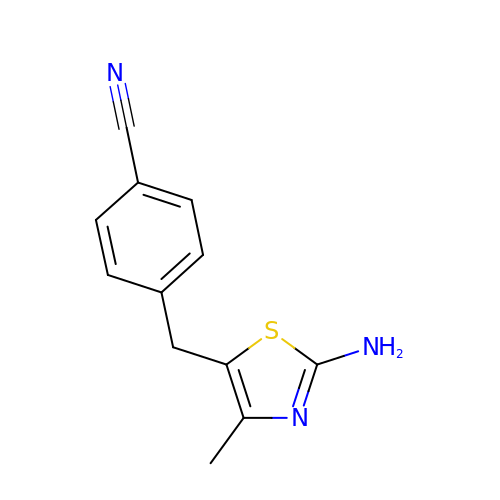4-[(2-azanyl-4-methyl-1,3-thiazol-5-yl)methyl]benzenecarbonitrile | C12 H11 N3 S | GRAVLCQUTREOOB-UHFFFAOYSA-N> SMPDEVPLDEQCERLPYDASKWEFARERLKLGKSLGRGAFGKVVQASAFGIKKSPTCRTVAVKMLKEGATASEYKALMTELKILTHIGHHLNVVNLLGACTKQGGPLMVIVEYCKYGNLSNYLKSKRDLFFLNKDAALHMEPKKEKMEPGLEQGKKPRLDSVTSSESFASSGFQEDKSLSDVEEEEDSDGFYKEPITMEDLISYSFQVARGMEFLSSRKCIHRDLAARNILLSENNVVKICDFGLARDIYKNPDYVRKGDTRLPLKWMAPESIFDKIYSTKSDVWSYGVLLWEIFSLGGS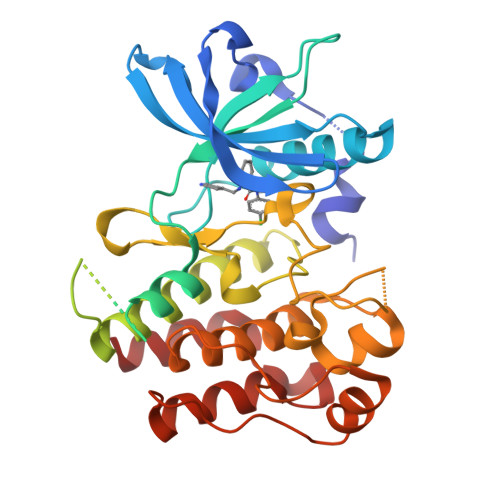PYPGVQMDEDFCSRLREGMRMRAPEYSTPEIYQIMLDCWHRDPKERPRFAELVEKLGDLL> SNAQSQSNQATPSKVVSGEVNAASFAQFSNAFIDDLWQLSPTWALYSGKHVNDGYLEIPDEAGRVKTLAFVKAQQAKLKQFELKSLTSNETIDYHLIDNLLSSMAWDITRFKSWQWDPSSYNVAGGFAQIINENFAPLDDRLRSVLARMENIPAYYAAARGNISQPTLEHTELAVLQNQGAFSVFSDDLLKQVADSGLSDAEKALFKTRFDIASKAINEHISWLNAQVSQLKKEGARSFRIGEELYEQKFAFDIQAGMTAKQLYQKAMVDKDRVQGEMAKITDKLWPKYFTTPKPSDNKIAIRQLIDKLSTK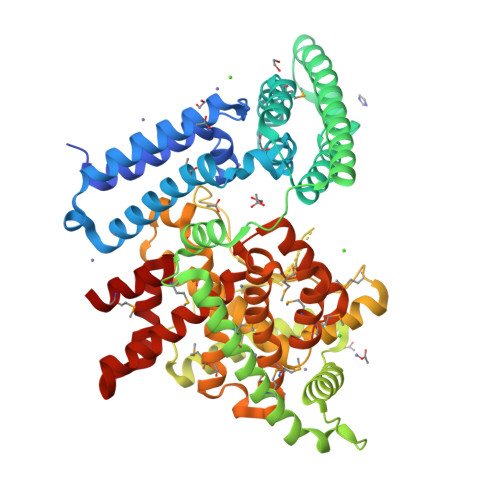HVKRDDFVSEVRKQIPELIEFVNQKNIVTLDPKKPLVVRETPEYMRGYASISAPGPYDKLGNTYYNVTPLDGMSNESAESYLREYNHWILQILNIHEAIPGHYTQLVYSNESPSLVKSLFGNGAMVEGWAVYTERMMLEEGYGNFEPEMWLMYYKWNLRVICNTILDYSIHVKGMTEEQAIALMMDEAFQQRAEAEGKWRRATLSQVQLTSYYSGYREIYDFREEYKQLKGKDFDLKAFHEKFLSYGSAPVKYIRQLMLE>[30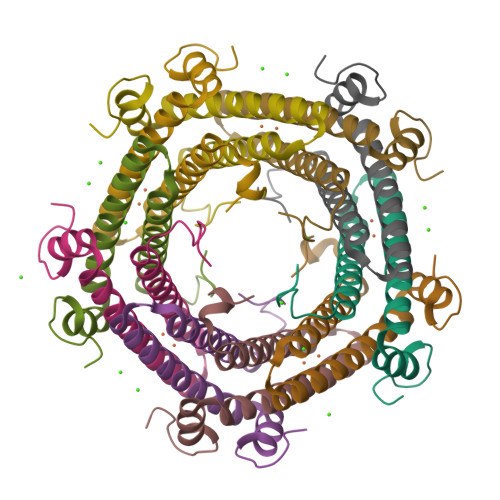x]MAQSSNSTHEPLEVLKEETVNRHRAIVSVMAELEAVDWYDQRVDASTDPELTAILAHNRDEEKEHAAMTLEWLRRNDAKWAEHLRTYLFTEGPITAANSSSVDKLAAALEHHHHHH MINDY1 and MINDY2 are members of the MINDY family of deubiquitinases (DUBs) that have exquisite specificity for cleaving K48-polyUb, yet we have a poor understanding of their catalytic mechanism. Here, we analyze the crystal structures of MINDY1 and MINDY2 alone and in complex with monoUb, di-, and penta-K48-polyUb, identifying 5 distinct Ub binding sites in the catalytic domain that explain how these DUBs sense both Ub chain length and linkage type to cleave K48-polyUb chains. The activity of MINDY1/2 is inhibited by the Cys-loop, and we find that substrate interaction relieves autoinhibition to activate these DUBs. We also find that MINDY1/2 use a non-canonical catalytic triad composed of Cys-His-Thr.

Despite this distance, we found a water molecule to coordinate T335 with H319 via hydrogen bonding, an unusual mechanism that may serve to orient H319 for catalysis, thereby adopting the function of the third catalytic residue. To test whether such an unusual catalytic architecture is possible, we introduced a T335V mutation to disrupt this water bridge, which resulted in a substantial loss of activity. As T335 serves a catalytic function to correctly position H319 for catalysis, we wondered if mutating T335 to a negatively charged residue would enhance the activity of MINDY1. To our surprise, the mutation of T335 to aspartate also abolishes MINDY1 activity. To understand the reason underlying this loss of activity, we determined the crystal structure of MINDY1T335D, which revealed the formation of an ionic interaction between T335D and the catalytic H319. H319 is locked in this conformation, which is further rigidified by the network of hydrogen bonds with Q131, S321, and N134, resulting in the catalytic Cys being rotated away from H319. Hence, the mutation T335D also forces the enzyme into an unproductive catalytic state, thus highlighting the requirement of a water molecule to bridge an interaction with T335 via hydrogen bonding to correctly position H319.

> GPLGSPEFPGRLEMEPDFYCVKWIPWKGEQTPIITQSTNGPCPLLAIMNILFLQWKVKLPPQKEVITSDELMAHLGNCLLSIKPQEKSEGLQLNFQQNVDDAMTVLPKLATGLDVNVRFTGVSDFEYTPECSVFDLLGIPLYHGWLVDPQSPEAVRAVGKLSYNQLVERIITCKHSSDTNLVTEGLIAEQFLETTAAQLTYHGLCELTAAAKEGELSVFFRNNHFSTMTKHKSHLYLLVDDQGFLQEEQVVWESLHNVDGDSCFCDSDFHLSHSLGKGPGAEGGSGSPE>MIDTLKNIKVKDVMTKNVITAKRHEGVVEAFEKMLKYKISSLPVIDDENKVI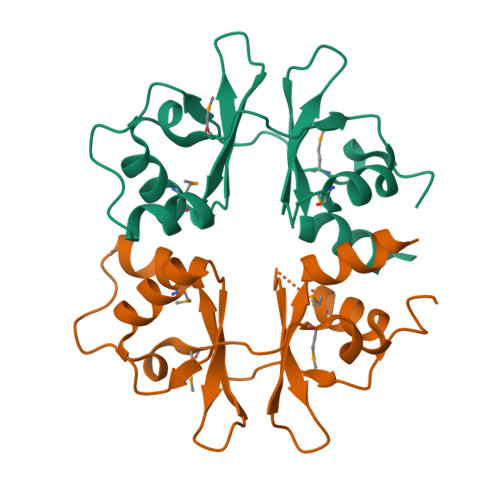GIVTTTDIGYNLIRDKYTLETTIGDVMTKDVITIHEDASILEAIKKMDISGKKEEIINQLPVVDKNNKLVGIISDGDIIRTISKII[4x]>[4x]MGSSHHHHHHS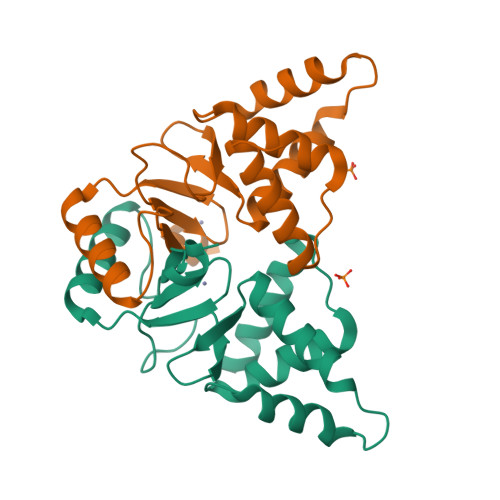QGSTAPHHHVDDANSFVRAVERACSERGLRLTPIRANVLRLIADAGKPVKAYELLDWVREGKGVGADAPPTVYRALDFLMANGFVHKLESVNAFVACHHPNSAQHSVPFLICDRCHSAVELEDRDVVSQLEARAKALGFQPQAQTLEVHGLCAKCAAAG In this study, we determined the co-crystal structures of drimenol synthase from Aquimarina spongiae (AsDMS), which catalyzes the conversion of farnesyl pyrophosphate (1) into drimenol (2). Crystallographic analyses of the enzyme bound to substrates 1 and drimenyl monophosphate (3) demonstrated that the TCβ domain catalyzes a class II cyclization reaction initiated by protonation, whereas the HAD domain catalyzes a phosphatase-like dephosphorylation reaction dependent on a divalent metal. Our results demonstrate that AsDMS is a bifunctional dimeric enzyme, comprising a protonation-initiated sesquiterpene cyclase (TCβ) domain and a metal-dependent HAD domain responsible for the stepwise release of phosphate to produce compound 2. The crystal structure revealed that AsDMS consists of N-terminal HAD and C-terminal TCβ domains connected by a highly flexible, disordered linker.

Because wild-type AsDMS possesses a long disordered region at its N-terminus, we truncated 18 residues from the N-terminus to generate AsDMS d18. Additionally, to obtain a co-crystal structure with substrate 1, we introduced the D333N mutation into AsDMS d18 (AsDMS d18/D333N), which abolished the protonation-initiated cyclization reaction. We determined the crystal structure of AsDMS d18/D333N at 2.30 Å resolution. The HAD domain comprised a Cap lobe and a Rossmann fold lobe. The asymmetric unit of the crystal structure contained two AsDMS molecules. Gel filtration analysis was conducted to evaluate the oligomeric state of AsDMS and confirmed that the major peak corresponded to the dimer. These results suggested that AsDMS forms a dimeric structure with a C2 symmetry axis. The obtained crystal structure of AsDMS represents the first experimentally determined structure of a HAD-TCβ enzyme, revealing distinct substrate-binding pockets for the HAD and TCβ domains. Among the top 20 identified proteins, only AsDMS exhibited structural differences within the core region of the Rossmann fold, notably lacking the conventional C-terminal α-helix involved in typical folding and instead possessing an additional N-terminal α-helix. In the monomeric state, the domain pockets are oriented back-to-back.

>[2x]GSHLTPELITSLQELSQILDRYDTIVFDLGDVLLHWDSVHFTSETKGIDDVRKMVKHPVWQDLEKGLINQEFALTALSCELETPCSKLKEMLELSIASLQVNPLMVEVLRVLHKKDKQIYCLSNVDLESFSYLYKQFDFWKYFDGIYVSALLQLRKPNPDIFQYLISSASINTKSTIFIDDKSENLQEAANFGISTLKYNKDNFEYTAIEGGWPIPLQNMTPEIHKKRTLGEDYLNLRLRKFPFCKSFVSNNVELIGGEDFSKEIFSTAVILHSYTSLPDDIIASMCHEILNHDGQNKLRWCFYKNEARPDNFPDDLNTTSMVLSFLLNHNKLTIEKIIPVAEQMIANRNEEGIIQVYFDDNRPRIDAIVAINVLYLMHQIGYGERKELKETEAFVFDFLISKEYLKGTRYYPAPDVFLFFLSRLVVDFPDQFEKFHKPLTEMLITRVNCSTFPLERALRIIALKKLGIVNRVDFLKLLDTQLADGGWPVYGLFIAPRSNTYFGSRELSTAFALEALHILS>VSEIKTLVTFFGGTGDLAKRKLYPSVFNLYKKGYLQKHFAIVGTARQALNDDEFKQLVRDCIKDFTDDQAQAEAFIEHFSYRAHDVTDAASYAVLKEAIEEAADKFDIDGNRIFYMSVAPRFFGTIAKYLKSEGLLADTGYNRLMIEKPFGTSYDTAAELQNDLENAFDDNQLFRIDHYLGKEMVQNIAALRFGNPIFDAAWNKDYIKNVQVTLSEVLGVEERAGYYDTAGALLDMIQNHTMQIVGWLAMEKPESFTDKDIRAAKNAAFNALKIYDEAEVNKYFVRAQYGAGDSADFKPYLEELDVPADSKNNTFIAGELQFDLPRWEGVPFYVRSGKRLAAKQTRVDIVFKAGTFNFGSEQEAQEAVLSIIIDPKGAIELKLNAKSVEDAFNTRTIDLGWTVSDEDKKNTPEPYERMIHDTMNGDGSNFADWNGVSIAWKFVDAISAVYTADKAPLETYKSGSMGPEASDKLLAANGDAWVFK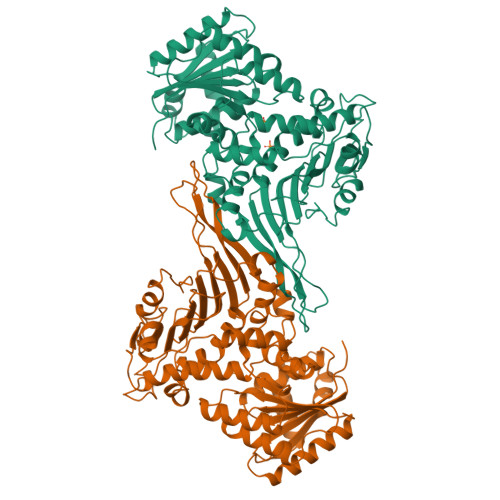G[2x]> GICKSSDCIKSAARLIQNMDATTEPCTDFFKYACGGWLKR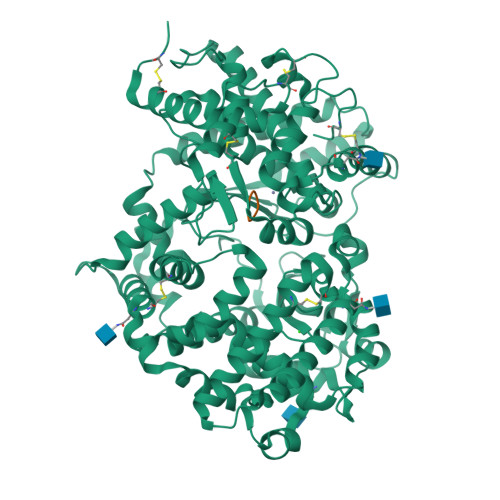NVIPETSSRYGNFDILRDELEVVLKDVLQEPKTEDIVAVQKAKALYRSCINESAIDSRGGEPLLKLLPDIYGWPVATENWEQKYGASWTAEKAIAQLNSKYGKKVLINLFVGTDDKNSVNHVIHIDQPRLGLPSRDYYECTGIYKEACTAYVDFMISVARLIRQEERLPIDENQLALEMNKVMELEKEIANATAKPEDRNDPMLLYNKMTLAQIQNNFSLEINGKPFSWLNFTNEIMSTVNISITNEEDVVVYAPEYLTKLKPILTKYSARDLQNLMSWRFIMDLVSSLSRTYKESRNAFRKALYGTTSETATWRRCANYVNGNMENAVGRLYVEAAFAGESKHVVEDLIAQIREVFIQTLDDLTWMDAETKKRAEEKALAIKERIGYPDDIVSNDNKLNNEYLELNYKEDEYFENIIQNLKFSQSKQLKKLREKVDKDEWISGAAVVNAFYSSGRNQIVFPAGILQPPFFSAQQSNSLNYGGIGMVIGHDITHGFDDNGRNFNKDGDLVDWWTQQSASNFKEQSQCMVYQYGNFSWDLAGGQHLNGINTLGENIADNGGLGQAYRAYQNYIKKNGEEKLLPGLDLNHKQLFFLNFAQVWCGTYRPEYAVNSIKTDVHSPGNFRIIGTLQNSAEFSEAFHCRKNSYMNPEKKCRVW;> AAAA>MEKNGNNRKLRVCVATCNRADYSKLAPIMFGIKTEPEFFELDVVVLGSHLIDDYGNTYRMIEQDDFDINTRLHTIVRGEDEAAMVESVGLALVKLPDVLNRLKPDIMIVHGDRFDALALATSAALMNIRILHIEGGEVSGTIDDSIRHAITKLAHYHVCCTRSAEQHLISMCEDHDRILLAGCPSYDKLLSAKNKDYMSIIRMWLGDDVKSKDYIVALQHPVTTDIKHSIKMFELTLDALISFNKRTLVLFPNIDAG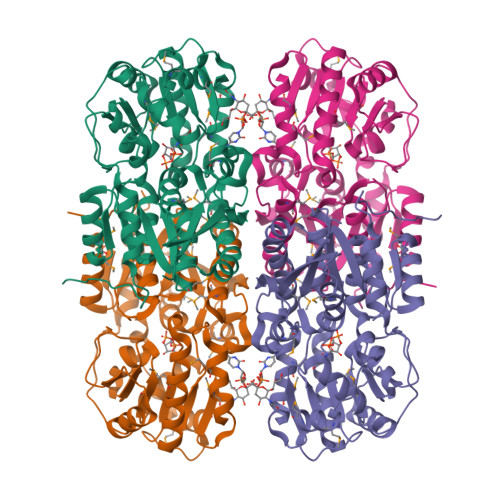SKEMVRVMRKKGIEHHPNFRAVKHVPFDQFIQLVAHAGCMIGNSSCGVREVGAFGTPVINLGTRQIGRETGENVLHVRDADTQDKILQALHLQFGKQYPCSKIYGDGNAVPRILKFLKSIDLQEPLQKKFCFPPVKENISQDIDHILEHHHHHH[4x]>[2x]SMELATMGKVNEVLFMNGGEGEISYAQNSSFTEKVASMAMPALENAVETLFSKDFHLLPALNAADLGCAAGPNTFAVISMIKRMMEKKCRELYCQTPELQVYLNDLFGNDFNTLFKGLSSEVVGNKCEEVSCYVMGVPGSFHGRLFPRNSLHLVHSSYSVHWLTQAPKGLTSR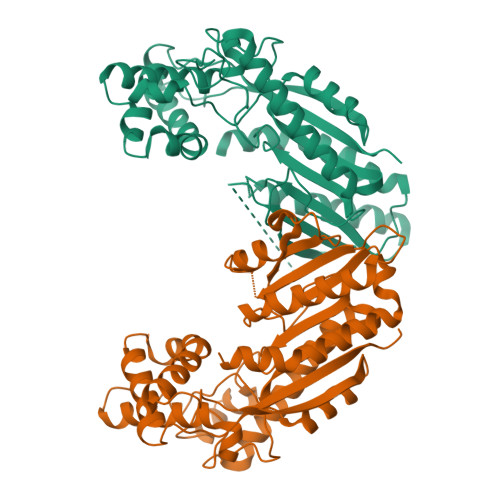EGLALNKGKIYISKTSPPAVKEAYLSQFHEDFTMFLNARSQEVVPNGCMVLILHGRQSSDPSEMESCFTWELLAIAIAELVSQGLIDEDKLDTFNVPSYFPSLEEVKDIVERDGSFTIDHLEGFELDSLEMQENDKWVRGDKFAKMVRAFTEPIISNQFGHEIMDKLYDKFTHIVVSDLEAELPKTTSIILVLSKIVG conserved and function as secondary active transporters. transport proteins that include the amino acid transporter LeuT18. μM range and that metal ion transport is coupled to the cotransport of protons. of the prokaryotic SLC11 transporter EcoDMT.

mutants of Glu129 and reduced to half in H236A. different role in proton-coupled metal ion transport. does not function as primary H+-acceptor. the pKa of Glu129 would have to be shifted upwards. in vicinity to the metal ion coordinating Asp51.

> MSETQSQTMTRPQDLSLSDINSTVEVPEGHSFWKTLLAYSGPGALVAVGYMDPGNWSTSITGGQNFQYLLLSIIVISSLLAMLLQNMAAKLGIVCQLDLAQAIRARTSRRLGFIFWILTELAIMATDIAQVIGAAIALYLLFKIPIFLAVVITVLDVFLLLLLNRIGFRKIEALVVCLIFVILFVFLYQIILSQPAWHQVAKGLIPSWASVQTSPKIGGQTPLSASLGIIGATIMPHNLFLHSAISQSRKIDRTDSSKVAEAVRFSNWDSNIQLSLAMVVNALLLIMGVAVFKSGAVQDPSFFGLYQALSNPDMVSNPVLAEAARSGVLSTLFAVALLASGQNSTITGTITGQVIMEGFIHLRLPLWLRRLVTRLIAIIPVVVCVAITSHQGSLDEHQALNNLMNNSQVFLALALPFSIVPLLMLTDSAAQMGNQFKNTRWVKVMGWLTVIILTLLNLISISSQIAGFFGDNPSSQDLLLSQVISIGIILAMIGLLIWTIIDIRRFTHPKQKALEVLFQ> ESRTKPFTVPILTVEEMTNSRFPIPLEKLFTGPSSAFVVQPQNGRCTTDGALLGTTQLSPVDICTFRGDVTHIAGTQNYTMNLASQNWNNYDPTEEIPAPLGTPDFVGKIQGVLTQTTRRDGSTRGHKATVSTGSVHFTPKLGSVQFSTDTSNDFETGQNTRFTPVGVVQDGSTTHQNEPQQWVLPDYSGRDSHNVHLAPAVAPTFPGEQLLFFRSTMPGCSGYPNMNLDCLLPQEWVQH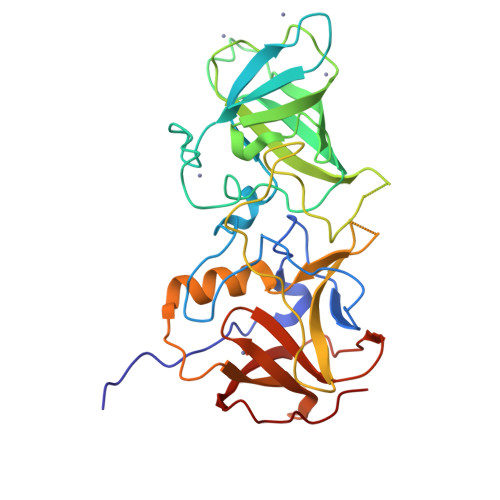FYQESAPAQSDVALLRFVNPDTGRVLFECKLHKSGYVTVAHTGQHDLVIPPNGYFRFDSWVNQFYTLAPMG>[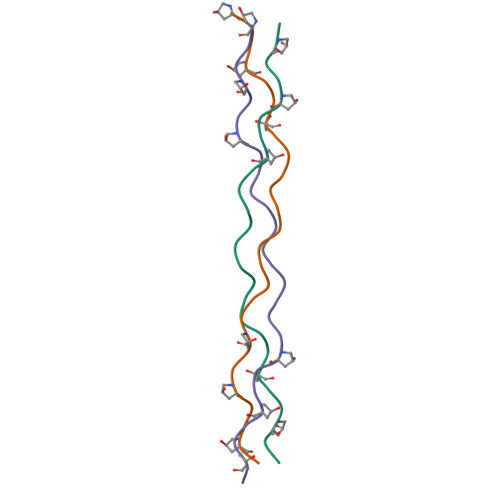6x]PPGPPGPPGPKGDQGEKGPPGPPGPPG Von Willebrand factor (VWF) assembly begins in the endoplasmic reticulum of endothelial cells and megakaryocytes where VWF is synthesized as a precursor with multiple domains. The polypeptide including the propeptide and mature VWF chain (proVWF) subsequently forms “tail-to-tail” homodimers through their C-terminal cystine knot (CK) domains. These proVWF dimers are then transported to the Golgi where they assemble into large multimers ‘head-to-head’ through interchain disulfide bonds between D3 domains of two proVWF dimers. Therefore, the disulfide linkages and the cysteines involved in the VWF D′D3 dimer interface remain to be confirmed with the discrepancy mainly on Cys1097 and Cys1099. Here we identified the disulfide linkages from the D′D3 dimer interface through chemical digestion and mass spectrometry and solved the cryo-electron microscopy (cryo-EM) structure of VWF tubules with each repeating unit containing one D′D3 dimer and one D1D2 dimer.

In order to gain further structural information of the D′D3 dimer interface, we purified D′D3 dimers complexed with D1D2 derived from the expression medium of HEK293 cells transfected with expression plasmid of D1D2D′D3-wt or D1D2D′D3-R1136M-E1143M. The tubule-like oligomers of these complexes were analyzed by single-particle cryo-EM. This yielded an electron density map covering two repeating units for D′D3-R1136M-E1143M dimer complexed with D1D2 at 3.3 Å resolution and an electron density map covering one repeating unit for D′D3-wt dimer complexed with D1D2 at 3.4 Å resolution respectively. Each repeating unit contains a D′D3 dimer and a D1D2 dimer. As the overall configuration of the refined D′D3-wt complex is essentially the same as that of the D′D3-R1136M-E1143M mutant, the structure of the mutant was selected for presentation due to its slightly better resolution. The shape of the repeating unit largely resembles that of MUC2 where a D′D3 dimer is docked in the central hole of the donut-shaped D1D2 dimer8. The connecting loop linking two helices in the D′D3 monomer restrained by the Cys1091–Cys1097 disulfide is anchored in a hydrophobic pocket formed by Phe1100, Met1055, and Val1056 through Ile1094, but in the dimer, it is more flexible with the intramolecular Cys1091–Cys1099 bond and flips over to dock in the same hydrophobic surface pocket of the other D′D3 molecule in a domain swapping-like fashion. This brings two Cys1097 residues in proximity and the subsequent formation of an intermolecular disulfide bond. As there are very limited noncovalent interactions in the D′D3 dimeric interface, D1D2 is indispensable for its dimerization by aligning two D3 monomers in optimal positions for their intermolecular disulfide formation.

>AEGTRGRSSTARCSLFGSDFVNTFDGSMYSFAGYCSYLLAGGCQKRSFSIIGDFQNGKRVSLSVYLGEFFDIHLFVNGTVTQGDQRVSMPYASKGLYLETEAGYYKLSGEAYGFVARIDGSGNFQVLLSDRYFNKTCGLCGNFNIFAEDDFMTQEGTLTSDPYDFANSWALSSGEQWCERASPPSSSCNISSGEMQKGLWEQCQLLKSTSVFARCHPLVDPEPFVALCEKTLCECAGGLECACPALLEYARTCAQEGMVLYGWTDHSACSPVCPAGMEYRQCVSPCARTCQSLHINEMCQERCVDGCSCPEGQLLDEGLCVESTECPCVHSGKRYPPGTSLSRDCNTCICRNSQWICSNEECPGECLVTGQSHFKSFDNRYFTFSGICQYLLARDCQDHSFSIVIETVQCADDRDAVCTRSVTVRLPGLHNSLVKLKHGAGVAMDGQDVQLPLLKGDLRIQHTVTASVRLSYGEDLQMDWDGRGRLLVKLSPVYAGKTCGLCGNYNGNQGDDFLTPSGLAEPRVEDFGNAWKLHGDCQDLQKQHSDPCALNPRMTRFSEEACAVLTSPTFEACHRAVSPLPYLRNCRYDVCSCSDGRECLCGALASYAAACAGRGVRVAWREPGRCELNCPKGQVYLQCGTPCNLTCRSLSYPDEECNEACLEGCFCPPGLYMDERGDCVPKAQCPCYYDGEIFQPEDIFSDHHTMCYCEDGFMHCTMSGVPGSLLPDAVLSSPLSHRSKR[2x];>[2x]SLSCRPPMVKLVCPADNLRAEGLECTKTCQNYDLECMSMGCVSGCLCPPGMVRHENRCVALERCPCFHQGKEYAPGETVKIGCNTCVCQDRKWNCTDHVCDATCSTIGMAHYLTFDGLKYLFPGECQYVLVQDYCGSNPGTFRILVGNKGCSHPSVKCKKRVTILVEGGEIELFDGEVNVKRPMKDETHFEVVESGRYIILLLGKALSVVWDRHLSISVVLKQTYQEKVCGLCGNFDGIQNNDLTSSNLQVEEDPVDFGNSWKVSSQCADTRKVPLDSSPATCHNNIMKQTMVDSSCRILTSDVFQDCNKLVDPEPYLDVCIYDTCSCESIGDCACFCDTIAAYAHVCAQHGKVVTWRTATLCPQSCEERNLRENGYECEWRYNSCAPACQVTCQHPEPLACPVQCVEGCHAHCPPGKILDELLQTCVDPEDCPVCEVAGRRFASGKKVTLNPSDPEHCQICHCDVVNLTCEACQEPGGLVVPPHHHHHH>MAHHHHHHMSANTELDLHSALAWPFFEPRHRELAAGIEAWCRANLAHEDHEDVDATCRRLVRELGAAGWLKYGVGGVAYGGHGDTIDTRAVCLLRETLAKHSGLADFALAMQGLGSGAISLGGTHEQKTRYLPRVANGTAIAAFALSEPEAGSDVAAMTLSAREDGDAYVLDGDKTWISNGGIADFYVVFARTGEAPGARGISAFVVDADTPGLEIAERIDVIAPHPLARLHFAGARVPRSQMLGAPGEGFKLAMR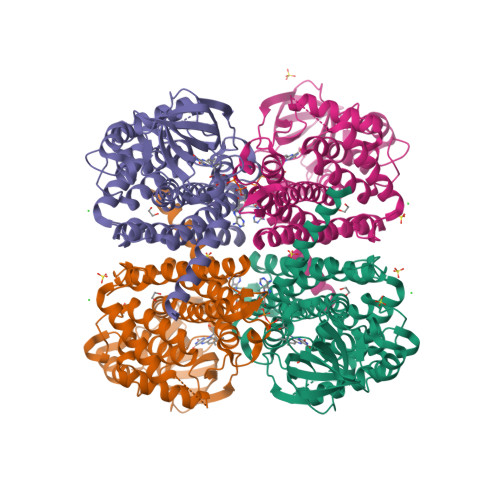TLDIFRTSVAAASLGFARHAMAEGVARAASRKMFGQTLGDFQLTQAKLAQMALTIDSSALLVYRAAWLRDQGENVTREAAMAKWHASEGAQQVIDAAVQLYGGMGVQSGTAVEMLYREIRALRIYEGATEVQQLIVGRDLLKAHAAATAGANTR[4x]>[2x]G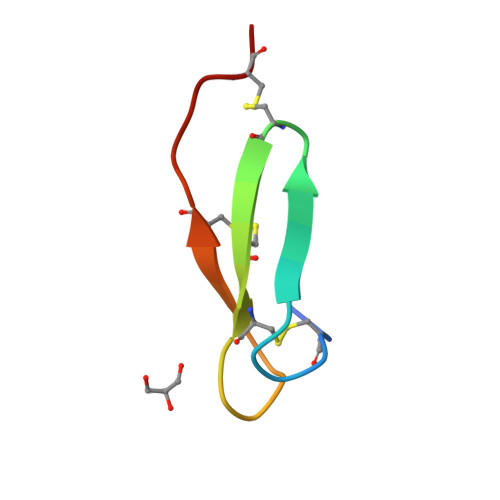SSCQPGTTFRRDCNTCVCNRDGTNAACTLRACL> TAR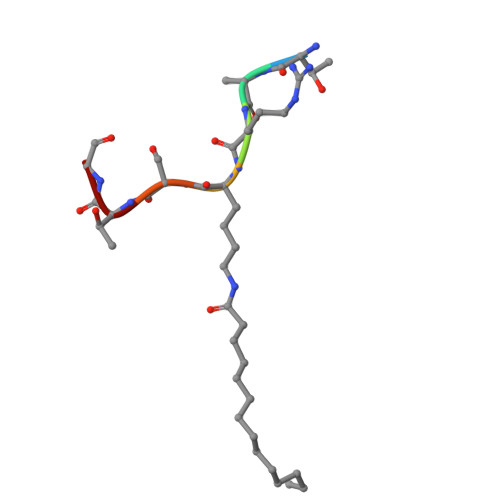XSTG> NKYG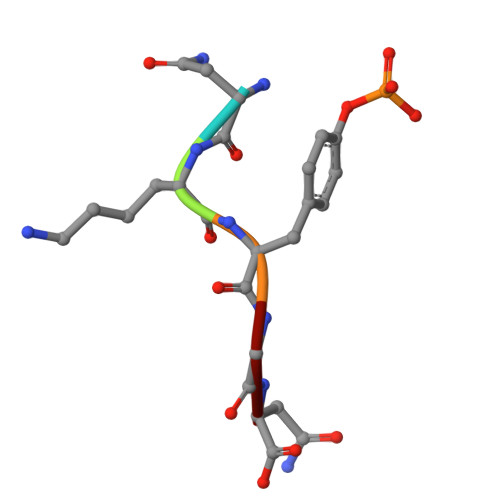N>MILIRGLTRVITFDDQERELEDADILIDGPKIVAVGKDLSDRSVSRTIDGRGMIALPGLINSHQHLYEGAMRAIPQLERVTMASWLEGVLTRSAGWWRDGKFGPDVIREVARAVLLESLLGGITTVADQHLFFPGATADSYIDATIEAATDLGIRFHAARSSMTLGKSEGGFCDDLFVEPVDRVVQHCLGLIDQYHEPEPFGMVRIALGPCGVPYDKPELFEAFAQMAADYDVRLHTHFYQPLDAGMSDHLYGMTPWRFLEKHGWASDRVWLAHAVVPPREEIPEFADAGVAIAHLIAPDLRMGWGLAPIREYLDAGITVGFGTTGSASNDGGNLLGDLRLAALAHRPADPNEPEKWLSARELLRMATRGSAECLGRPDLGVLEEGRAADIACWRLDGVDRVGVHDPAIGLIMTGLSDRASLVVVNG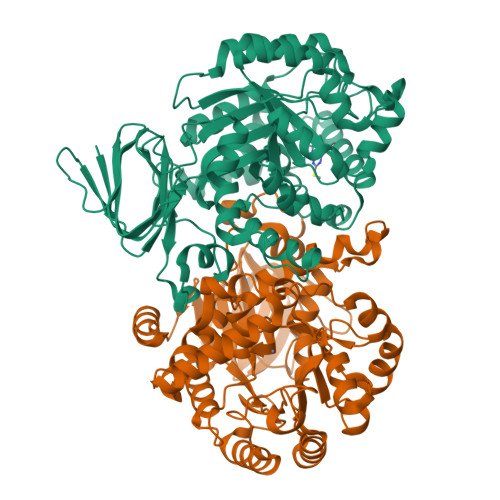QVLVENERPVLADLERIVANTTALIPKNL[2x]> GSSSKPTDRGQQYKDGKFTQPFSLVNQPDAVGAPINAGDFAEQINHIRNSSPRLYGNQSNVYNAVQEWLRAGGDTRNMRQFGIDAWQMEGADNYGNVQFTGYYTPVIQARHTRQGEFQYPIYRMPPKRGRLPSRAEIYAGALSDKYILAYSNSLMDNF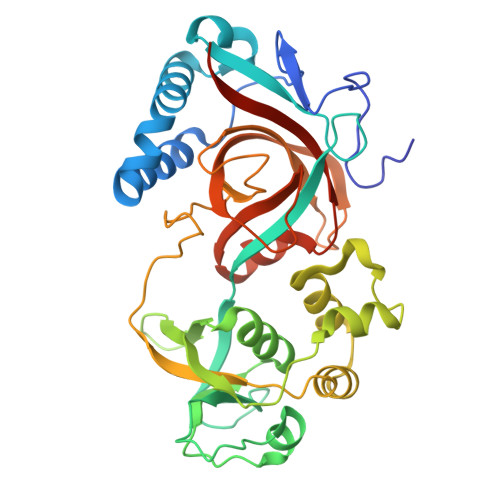IMDVQGSGYIDFGDGSPLNFFSYAGKNGHAYRSIGKVLIDRGEVKKEDMSMQAIRHWGETHSEAEVRELLEQNPSFVFFKPQSFAPVKGASAVPLVGRASVASDRSIIPPGTTLLAEVPLLDNNGKFNGQYELRLMVALDVGGAIKGQHFDIYQGIGPEAGHRAGWYNHYGRVWVLKTAPGAGNVFSG>[2x]SAVRPTKRIEFTEADGDTEGKSVFQLEKETDKETFKIRD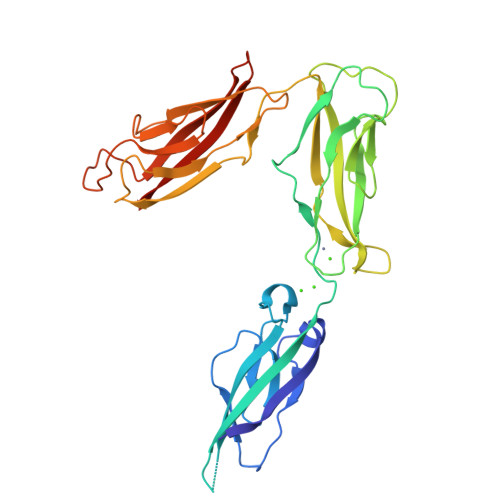DNPWVTVETNGAVRVKKKWDYEELGPEKTIDFWVIITNMGHNAGIKYTDNQRVIILVKDVNDEPPYFINRPLPMQAVVQLNAPPNTPVFTLQARDPDTDHNIHYFIVRDRTGGRFEVDERSGVVRTRGTDLFQLDMEYVLYVKAEDQNGKVDDRRFQSTPEERLSIVGGKRAPQFYMPSYEAEIPENQKKDSDIISIKAKSFADREIRYTLKAQGQGAGTFNIGPTSGIVKLAKELDFEDLRQPHVYSLIVTATEDSGGFSTSVDLTIRVTDVNDNA> MAVTLDKDAYYRRVKRLYSNWRKGEDEYANVDAIVVSVGVDEEIVYAKSTALQTWLFGYELTDTIMVFCDDKIIFMASKKKVEFLKQIANTKGNENANGAPAITLLIREKNESNKSSFDKMIEAIKESKNGKKIGVFSKDKFPGEFMKSWNDCLNKEGFDKIDISAVVAYTIAVKEDGELNLMKKAASITSEVFNKFFKERVMEIVDADEKVRHSKLAESVEKAIEEKKYLAGADPSTVEMCYPPIIQSGGNYNLKFSVVSDKNHMHFGAITCAMGIRFKSYCSNLVRTLMVDPSQEVQENYNFLLQLQEELLKELRHGVKICDVYNAVMDVVKKQKPELLNKITKNLGFGMGIEFREGSLVINSKNQYKLKKGMVFSINLGFSDLTNKEGKKPEEKTYALFIGDTVLVDEDGPATVLTS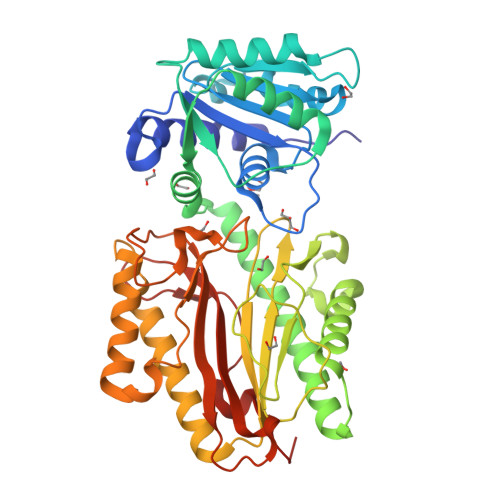VKKKVKNVGIFLKN2-[[2-fluoranyl-4-(3-methoxyphenyl)phenyl]carbamoyl]cyclopentene-1-carboxylic acid | C20 H18 F N O4 | 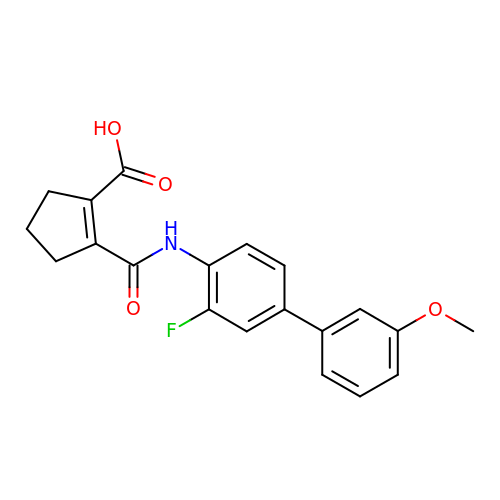XPRDUGXOWVXZLL-UHFFFAOYSA-N>MTKKLIKEVALTLFAEKGYDGTALSEIAKAVGIKTPSLYAHFASKEALFLEVYQDSIQMELTELGRVAEREDLVGEEKLQSIFFVATDFSSNPDEKKFFQRAVFYP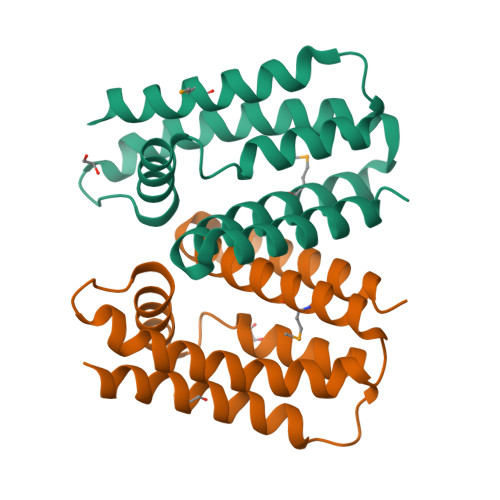PKSLFQELKEETKTYEQLTNRILRETLEKIVSEEALVRWMHVFYALLDGLSVEHGIYDETEFELRRKSAWAVLASLLK[2x]>[4x]SNADVTPLSLGIETLGGIMTKLITRNTTIPTKKSQVFSTAADGQTQVQIKVFQGEREMATSNKLLGQFSLVGIPPAPRGVPQVEVTFD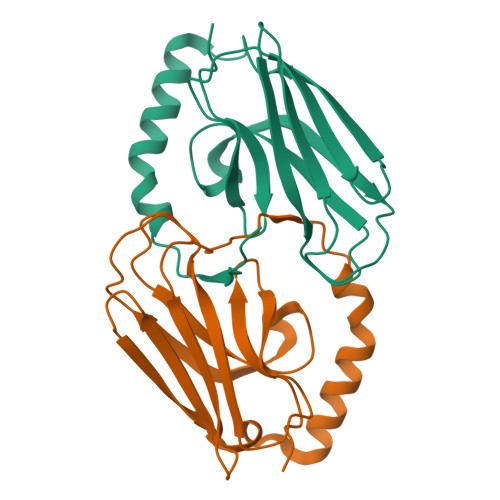IDANGIVNVSARDRGTGKEQQIVIQSSGGLSKDQIENMIKEAEKNAAEDAKRKELVEVINQAE> AATKQTA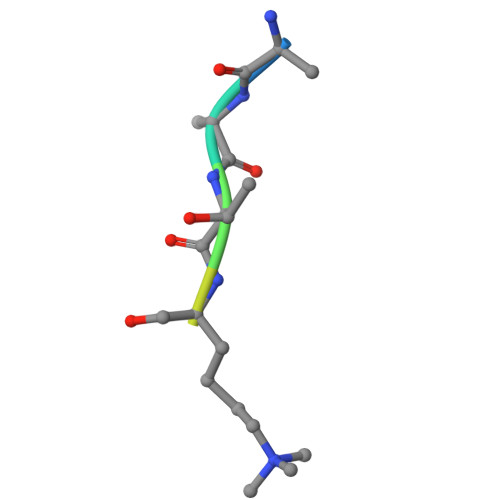R>GPLGSMGNSGFYLYNTENCVFADNIKVGQMTEPLKDQQIILGTKSTPVAAKMTASDGISLTVSNNS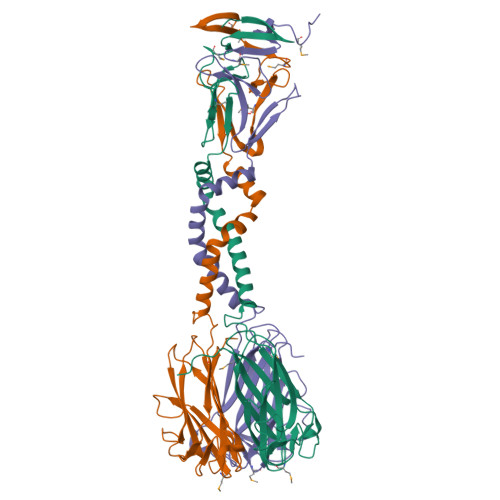STNASITIGLDAEKAYQLILEKLGNQILDGIADTIVDSTVQDILDKITTDPSLGLLKAFNNFPITNKIQCNGLFTPSNIETLLGGTEIGKFTVTPKSSGSMFLVSADIIASRMEGGVVLALVREGDSKPCAISYGYSSGVPNLCSLRTSITNTGLTPTTYSLRVGGLESGVVWVNALSNGNDILGITNTSNVSFLEVIPQTNA[6x]> GSHMFMPSDRSTERCETVLEGETISCFVVGGEKRLCLPQILNSVLRDFSLQQINAVCDELHIYCSRCTADQLEILKVMGILPFSAP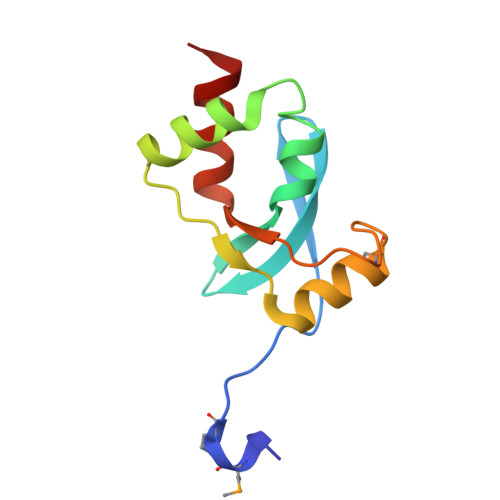SCGLITKTDAERLCNALLYG> GSHMQMVPPSAYDRAITVFSPEGRLYQVEYAREAVRRGTTAIGIACKDGVVLAVDRRITSKLVKIRSIEKIFQIDDHVAAATSGLVADARVLIDRARLEAQIYRLTYGEEISIEMLAKKICDIKQAYTQHGGVRPFGVSLLIAGIDKNEARLFETDPSGALIEYKATAIGSGRPV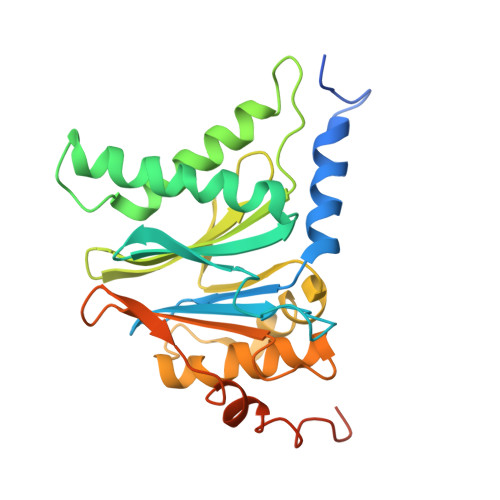VMELLEKEYRDDITLDEGLELAITALTKANEDIKPENVDVCIITVKDAQFKKIPVEEIKKLIEKVKKKLNEENKKEEENREETKEKQEE>[4x]MRVLVLLACLAAASNAGSQYETYQWDEDYDQEPDDDYQTGFPFRQNVDYGVPFHQYTLGCVSECFCPTNFPSSMYCDNRKLKTIPNIPMHIQQLYLQFNEIEAVTANSFINATHLKEINLSHNKIKSQKIDYGVFAKLPNLLQLHLEHNNLEEFPFPLPKSLERLLLGYNEISKLQTNAMDGLVNLTMLDLCYNYLHDSLLKDKIFAKMEKLMQLNLCSNRLESMPPGLPSSLMYLSLENNSISSIPEKYFDKLPKLHTLRMSHNKLQDIPYNIFNLPNIVELSVGHNKLKQAFYIPRNLEHLYLQNNEIEKMNLTVMCPSIDPLHYHHLTYIRVDQNKLKEPISSYIFFCFPHIHTIYYGEQRSTNGQTIQLKTQVFRRFPDDDDESEDHDDPDNAHESPEQEGAEGHFDLHYYENQEAAADYKDDDDK

SLRPs comprise an important family of proteins, divided into five subclasses, that influence collagen fibril formation. Recently, our group has demonstrated that Osteomodulin (OMD), a member of class II SLRPs, regulates the diameter and shape of collagen fibrils. In conclusion, we found that OMD binds to type-I collagen driven by weak electrostatic forces involving the residues Glu284 and Glu303 of a conspicuously, negatively charged patch of the protein. The weak nature of these interactions and the fast association and dissociation rates suggest that OMD shuttles on and off the growing collagen fibril in a fast-equilibrium.

Because SLRPs, and DCN in particular, have been described generally as dimeric proteins we first investigated the oligomeric state of OMD in solution by size-exclusion chromatography with multi-angle light scattering (SEC-MALS). Contrary to our expectations, the data indicated that the molecular weight of OMD was 54.7 kDa, a value consistent with a monomeric conformation in solution. To address this question, we determined the X-ray crystal structure of OMD at 2.17 Å resolution. The structure showed the typical curved solenoid fold characteristic of SLRPs displaying a large concave and convex surfaces. Despite the high concentration employed to crystalize the protein, OMD was found to be a monomer also in the crystalline state as demonstrated by the lack of stabilizing interactions and the small area of contact with neighboring protein chains in the crystal, as calculated with the PISA server. The structure of OMD was superimposed into the structure of DCN. The value of RMSD (calculated for the main chain alpha-carbons) was 1.3 Å, demonstrating that their overall fold was very similar. The difference in the dimerization propensity is explained by the lack of key intermolecular protein–protein interactions between neighboring units caused by variations in their amino acid sequence. OMD is an acidic (negatively charged) protein with a pI of 5.2, whereas collagen is a basic (positively charged) protein with a pI of 9. Considering that the main driving force of binding was electrostatic in nature (see above), we mapped the electrostatic surface of OMD in the crystal structure searching for negatively charged patches that could contribute to binding. We note that residues E284 and E303 located on the concave side near the C-terminal region of OMD are critical for binding, whereas the region near the N-terminal end do not seem to critically contribute to collagen binding as suggested from mutations L144W and Q145A.>MHELTIYHFMSDKLNLYSDIGNIIALRQRAKKRNIKVNVVEINETEGITFDECDIFFIGGGSDREQALATKELSKIKTPLKEAIEDGMPGLTICGGYQFLGKKYITPDGTELEGLGILDFYTESKTNRLTGDIVIESDTFGTIVGFENHGGRTYHDFGTLGHVTFGYGNNDE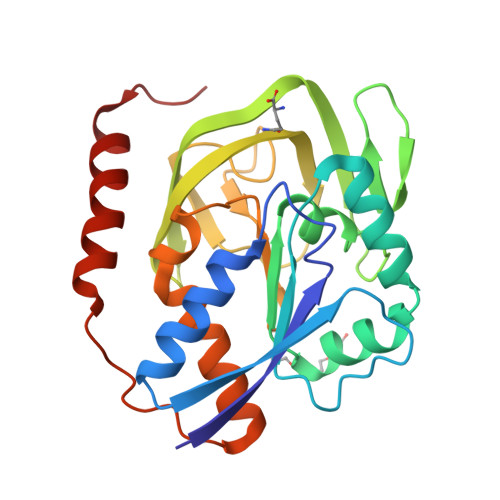DKKEGIHYKNLLGTYLHGPILPKNYEITDYLLEKACERKGIPFEPKEIDNEAEIQAKQVLIDRANRQKKSR[2x]>SGSGSTAEPDLKTALKAVIPAKRELFKQVKERSDEVIGEVKVANVIGGMRGLKSMLWEGSVLDPEEGIRFHGKTIKDCQKELPKGTSGTEMLPEAMFWLLLTGQVPSTNQVRAFSRELAEQSHLPQHILDLIKSFPRSMHPMTQLSIAVAALNTESKFAKAYEKGLSKADYWEPTFDDSISLLAKIPRVAALVFRPDEVDQVGTQALDASQDWSYNFAELLGKGGKENQDFHDLLRLYLALHGDHEGGNVSAHATHLVGSALSDPFLSYSAGLLGLAGPLHGLAAQEVLRWILAMQDKIGTKFTDDDVRNYLWDTLKSGRVVPGYGHAVLRKPDPRFQALMDFAATRPDVLANPVFQ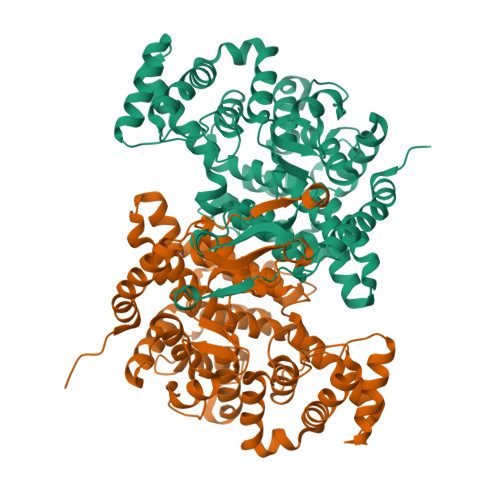LVKKNSEIAPAVLTEHGKTKNPHPNVDAASGVLFYHYGFQQPLYYTVTFGVSRALGPLVQLIWDRALGLPIERPKSINLLGLKK[4x]(10E,12Z)-hexadeca-10,12-dienal | C16 H28 O | 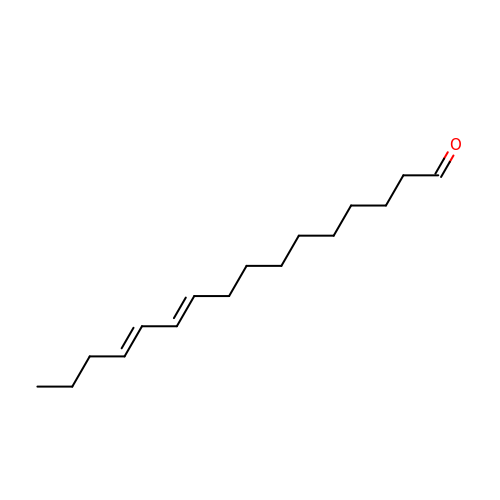OSFASEAZCNYZBW-SCFJQAPRSA-N> GNSTSSDKNNSSSEGNEGV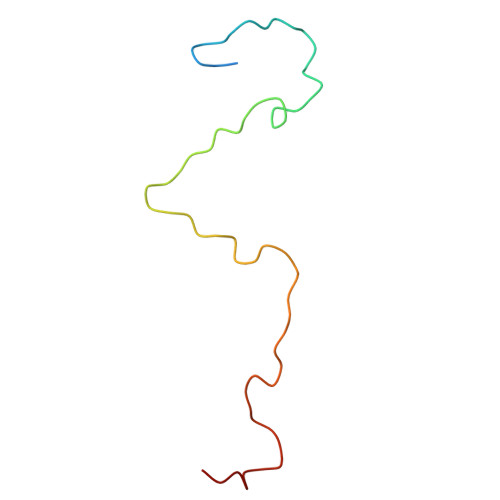IINNFYSNQYQNSIDLSANATGSDPPKTYGQFSNLLSGAVNAFSNMLPLLA>[2x]MGKVNVAKLRYMSRDDFRVLTAVEMGMKNHEIVPGSLIASIASLKHGGCNKVLRELVKHKLIAWERTKTVQGYRLTNAGYDYLALKTLSSRQVVESVGNQMGVGKESDIYIVA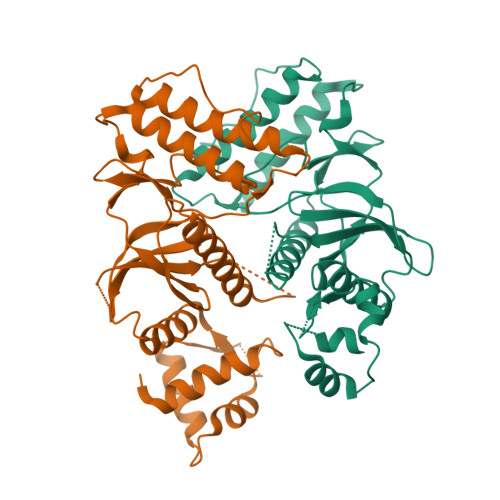NEEGQQFALKLHRLGRTSFRNLKNKRDYHKHRHNVSWLYLSRLSAMKEFAYMKALYERKFPVPKPIDYNRHAVVMELINGYPLCQIHHVEDPASVYDEAMELIVKLANHGLIHGDFNEFNLILDESDHITMIDFPQMVSTSHPNAEWYFDRDVKCIKDFFMKRFSYESELFPTFKDIRREDTLDVEVSASGYTKEMQADDELLHPLG> MIVKRPVSASLARAFFYIVL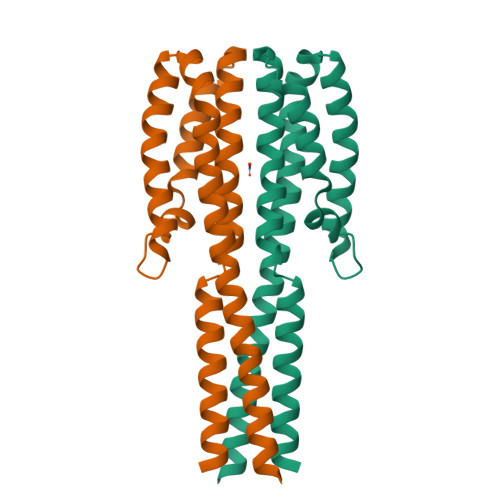LSILSTGIALLTLASSLRDAEAINIAGSLRMQSYRLGYDLQSGSPQLNAHRQLFQQALHSPVLTNLNVWYVPEAVKTRYAHLNANWLEMNNRLSKGDLPWYQANINNYVNQIDLFVLALQHYAERKMLLVVAISLAGGIGIFTLVFFTLRRIRHQVVAPLNQLVTASQRIEHGQFDSPPLDTNLPNELGLLAKTFNQMSSELHKLYRSLEHHHHHH> MNDIKQLLWNGELNVLVSIDPSFLMKGSPREIAVLRIRVPRETYLVNYMPLIWNKIKSFLSFDPLTDSEKYFWFEHNKTPIPWNYPVGVLFDCLAGKSATFTTSFENQVKDVLTFLRIHLVMGDSLPPTIIPIASSKTQAEKFWFHQWKQVCFILNGSSKAIMSLSVNEARKFWGSVITRNFQDFIEISNKISSSRPRHIPLIIQTSRTSGTFRISQPTISMTGVNPTLKDIEGDILDVKEGINGNDVMVICQGIEIPWHMLLYDLYSKLRSFDGFLYITLVPI;> GPHMGNFIITERKKAKEERSNPQTDSMDDLLIRRLTDRNDKEAHLNELF;> GAHMNIQKIQIKFQPIGSIGQLKPSVCKISMSQSFAMVILFLKRR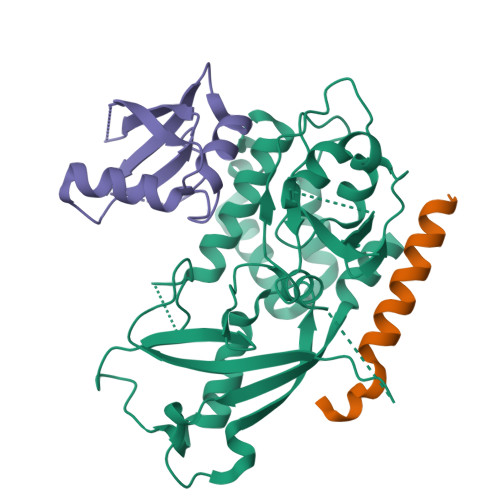LKMDHVYCYINNSFAPSPQQNIGELWMQFKTNDELIVSYCASVAFG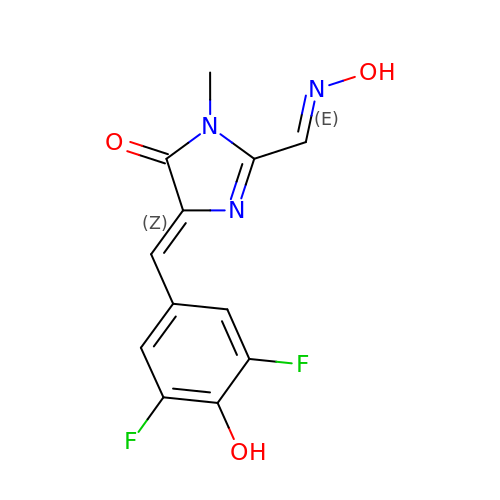(5Z)-5-[(3,5-difluoro-4-hydroxyphenyl)methylidene]-2-[(E)-(hydroxyimino)methyl]-3-methyl-3,5-dihydro-4H-imidazol-4-one | C12 H9 F2 N3 O3 | MZFHSQVSFUWKDU-TUUOAFJKSA-N> MLEKLNNINFNNISNNPNLGIEVGREIQNASWVKSPFFSITGTGADRGVRLFSVASQQPFRPRIKAQLTGSGVSGNTDFEANYDNLEILSQTIYPDAFGNSLRSKIK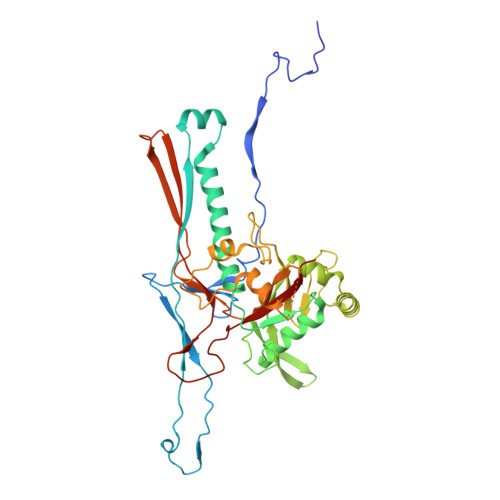AYSELERIDFIKESVDSLTTWMNEERDKRIVASLTNDFTNYLYNAAMNVATIRKAIFHARNGLKADNSKAFPIKPIRATMQSVGNVVVQNTSYIILLDSYQANQLKADSEFKELRKLYAFAGEDKGMLYSGLLGVIDNCPVIDAGVWNKLNVGMPNSSISDSDFTRYLNKANVSNIVTPMQLKEKLNQEKLNQEKLNQEKLKNKDISIGCLIGASAVLLAGSKETRFYIDETVDAGRKSLVGVDCLLGVSKARYQSTDGVVTPYDNQDYAVIGLVSNME> LCLSQQFKAQGDYILGGLFPLGSTEEATLNQRTQPNSIPCNRFSPLGLFLAMAMKMAVEEINNGSALLPGLRLGYDLFDTCSEPVVTMKSSLMFLAKVGSQSIAAYCNYTQYQPRVLAVIGPHSSELALITGKFFSFFLMPQVSYSASMDRLSDRETFPSFFRTVPSDRVQLQAVVTLLQNFSWNWVAALGSDDDYGREGLSIFSSLANARGICIAHEGLVPQHDTSGQQLGKVLDVLRQVNQSKVQVVVLFASARAVYSLFSYSIHHGLSPKVWVASESWLTSDLVMTLPNIARVGTVLGFLQRGALLPEFSHYVETHLALAADPAFCASLNAELDLEEHVMGQRCPRCDDIMLQNLSSGLLQNLSAGQLHHQIFATYAAVYSVAQALHNTLQCNVSHCHVSEHVLPWQLLENMYNMSFHARDLTLQFDAEGNVDMEYDLKMWVWQSPTPVLHTVGTFNGTLQLQQSKMYWPGNQVPVSQCSRQCKDGQVRRVKGFHSCCYDCVDCKAGSYRKHPDDFTCTPCNQDQWSPEKSTACLPRRPKFLAWGEPVVLSLLLLLCLVLGLALAALGLSVHHWDSPLVQASGGSQFCFGLICLGLFCLSVLLFPGRPSSASCLAQQPMAHLPLTGCLSTLFLQAAETFVESELPLSWANWLCSYLRGLWAWLVVLLATFVEAALCAWYLIAFPPEVVTDWSVLPTEVL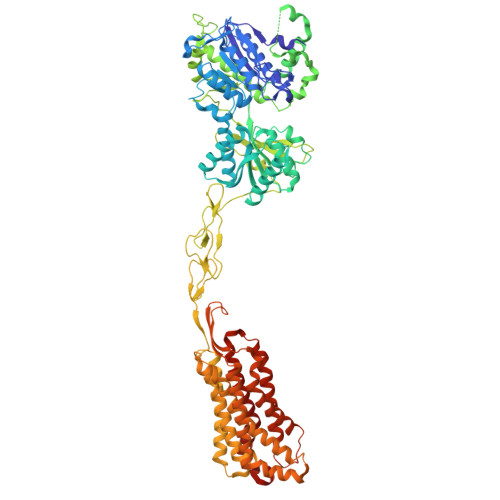EHCHVRSWVSLGLVHITNAMLAFLCFLGTFLVQSQPGRYNRARGLTFAMLAYFITWVSFVPLLANVQVAYQPAVQMGAILVCALGILVTFHLPKCYVLLWLPKLNTQEFFL>MEVEKTACPSGKKAREIDESLIFYKKWELEACVDAALLATQMDRVNAIPFTYEQLDVLKHKLDELYPQGYPESVIQHLGYLFLKMSPEDIRKWNVTSLETLKALLEVNKGHEMSPQVATLIDRFVKGRGQLDKDTLDTLTAFYPGYLCSLSPEELSSVPPSSIWAVRPQDLDTCDPRQLDVLYPKARLAFQNMNGSEYFVKIQSFLGHHHHHH[2x]

The tumor-associated antigen mesothelin is expressed at high levels on the cell surface of many human cancers, while its expression in normal tissues is limited. The binding of mesothelin to the tumor-associated cancer antigen 125 (CA-125) can lead to heterotypic cell adhesion and tumor metastasis within the pleural and peritoneal cavities. Here, we report the crystal structures of mesothelin that reveal a compact, right-handed solenoid consisting of 24 short helices and connecting loops. These helices form a nine-layered spiral coil that resembles ARM/HEAT family proteins.

Here, we report the crystal structures of a 207-residue MSLN fragment, of fl-MSLN alone and in complex with a therapeutic mAb MORAb-009, as well as the structure of its C-terminal shed-resistant peptide complexed with mAb 15B6. By truncation and alanine replacement mutagenesis, the CA-125 binding site was mapped to a 64-residue fragment at the N-terminus of MSLN. The N-terminal half of mesothelin is conformationally rigid, suitable for eliciting specific antibodies, whereas its C-terminal portion is more flexible.> MSFFRDLLESVVPTAYAEEPVEDVEVEQPEDAPEEEVSEETVEEEEEDDEDDDEDDEEEEETADPLDTLREECTKTAACKPFDHHFHECIERVTKEQEEPDYEHKHYKEDCIEEFFHLQH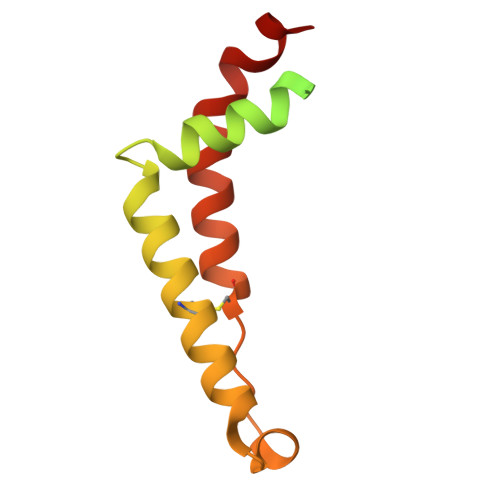CVNDCVAPRLFNRLK>DEDEDDLQRYIDV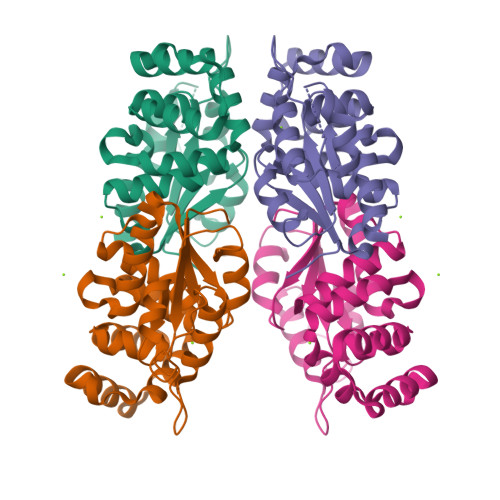TRGELFFARGIIFVEGDAERFLIPAFAEALDIHLDILGISVCSVSGTNFAPYIKLVGPTGLNIPHVVLTDLDPVDDRPPLARKRLLRLLELAVTDEEWDELDEDEPWDLGEEYGYFVNDSTLEPELFQAGLGSGIRDVIESELSTSAQTREALACWVDDPTALNNERLLKLIERIGKGRFAQALAGFATADTCPAYIRNALEYIRDAVALEHHHHHH[2x]>MGGAYETEKPTKDAAALETQSPEDFDQPSPLRKIISVASIAAGVQFGWALQLSLLTPYVQLLGIPHKWSSLIWLCGPVSGMIVQPIVGFHSDRCRSKFGRRRPFIATGAALVAVAVFLIGYAADFGYKMGDKLEEKVKVRAIGIFALGFWILDVANNTLQGPCRAFLADLAAGDAKRTRVANAFFSFFMAVGNVLGYAAGSYTNLHKMFPFTMTKACDIYCANLKTCFFLSITLLLIVTVTSLWYVNDKQWSPPPRNADDDEKTSSVPLFGEIFGAFKVMKRPMWMLLIVTALNWIAWFPFLLFDTDWMGREVFGGDSDGNERSKKLYSLGVQSGAMGLMFNSIVLGFMSLGVEWIGRKLGGAKRLWGIVNFILAAGLAMTVLVTKFAEDHRKTAGDLAGPSASVKAGALSLFAVLGI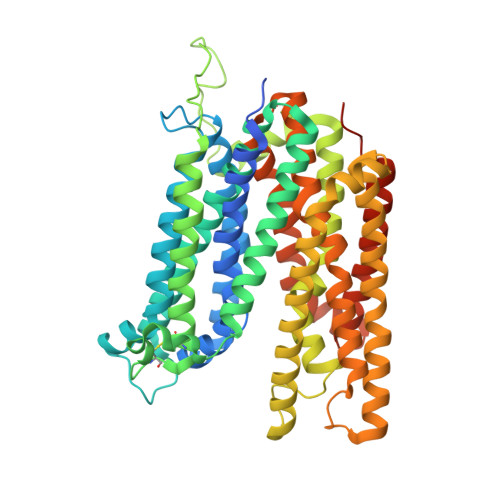PLAITFSTPFALASIFSSCSGAGQGLSLGVLNLAIVIPQMIVSLGGGPFDALFGGGNLPAFIVAAIAAAISGVLALTVLPSPPPDAPKATTMGGFHGLVPR[2x]> MSRSKRDNNFYSVEIGDSTFTVLKRYQNLKPIGSGAQGIVCAAYDAILERNVAIKKLSRPFQNQTHAKRAYRELVLMKCVNHKNIIGLLNVFTPQKSLEEFQDVYIVME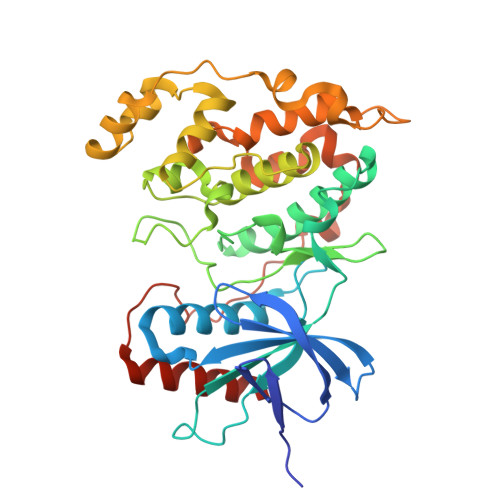LMDANLSQVIQMELDHERMSYLLYQMLCGIKHLHSAGIIHRDLKPSNIVVKSDATLKILDFGLARTAGTSFMMTPYVVTRYYRAPEVILGMGYKENVDIWSVGCIMGEMIKGGVLFPGTDHIDQWNKVIEQLGTPSPEFMKKLQPTVRTYVENRPKYAGYSFEKLFPDVLFPADSEHNKLKASQARDLLSKMLVIDASKRISVDEALQHPYINVWYDPSEAEAPPPKIPDKQLDEREHTIEEWKELIYKEVMDLEHHHHHH> GSSRGFPEDSEPISISHGNYTKQYPVFVGHKPGRNTTQRHRLDIQMIMIMNRTLYVAARDHIYTVDIDTSHTEEIYCSKKLTWKSRQADVDTCRMKGKHKDECHNFIKVLLKKNDDTLFVCGTNAFNPSCRNYRVDTLETFGDEFSGMARCPYDAKHANIALFADGKLYSATVTDFLAIDAVIYRSLGDSPTLRTVKHDSKWLKEPYFVQAVDYGDYIYFFFREIAVEYNTMGKVVFPRVAQVCKNDMGGSQRVLEKQWTSFLKARLNCSVPGDSHFYFNILQAVTDVIRINGRDVVLATFSTPYNSIPGSAVCAYDMLDIANVFTGRFKEQKSPDSTWTPVPDERVPKPRPGCCAGSSSLEKYATSNEFPDDTLNFIKTHPLMDEAVPSIINRPWFLRTMVRYRLTKIAVDNAAGPYQNHTVVFLGSEKGIILKFLARIGSSGFLNGSLFLEEMNVYNPEKCSYDGVEDKRIMGMQLDRASGSLYVAFSTCVIKVPLGRCERHGKCKKTCIASRDPYCGWVRESGSCAHLSPLSRLTFEQDIERGNTDGLGDCHN;> GTTGMPQYSTFHSENRDWTFNHLTVHRRTGAVYVGAINRVYKLTGNLTIQVAHKTGPEEDNKACYPPLIVQPCSEVLTLTNNVNKLLIIDYSENRLLACGSLYQGVCKLLRLDDLFILVEPSHKKEHYLSSVNKTGTMYGVIVRSEGEDGKLFIGTAVDGKQDYFPTLSSRKLPRDPESSAMLDYELHSDFVSSLIKIPSDTLALVSHFDIF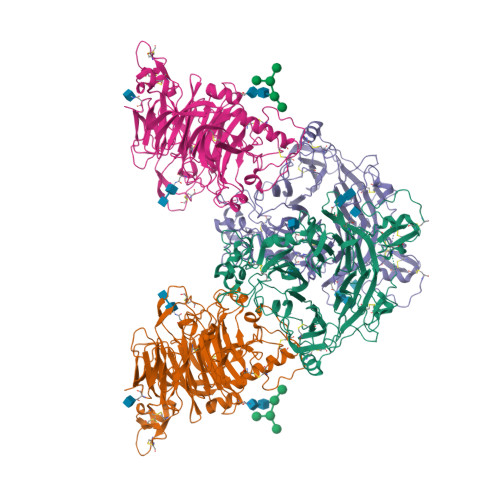YIYGFASGGFVYFLTVQPETPDGMAINSAGDLFYTSRIVRLCKDDPKFHSYVSLPFGCTRAGVEYRLLQAAYLAKPGEALAQAFNISSDEDVLFAIFSKGQKQYHHPPDDSALCAFPIRAINLQIKERLQSCYHGEGNLELNWLLGKDVQCTKAPVPIDDNFCGLDINQPLGGSTPVEGLTLYTTSRDRLTSVASYVYNGYSVVFVGTKSGKLKKIRADGPPHGGVQYEMVSVFKDGSPILRDMAFSINQLYLYVMSERQVTRVPVESCEQYTTCGECLSSGDPHCGWCALHNMCSRRDKCQRAWEANRFAASISQCMSSRENLYFQ N~2~-[(2R)-2-benzyl-3-(tert-butylsulfonyl)propanoyl]-N-{(1R)-1-(cyclohexylmethyl)-3,3-difluoro-2,2-dihydroxy-4-[(2-morpholin-4-ylethyl)amino]-4-oxobutyl}-3-(1H-imidazol-3-ium-4-yl)-L-alaninamide 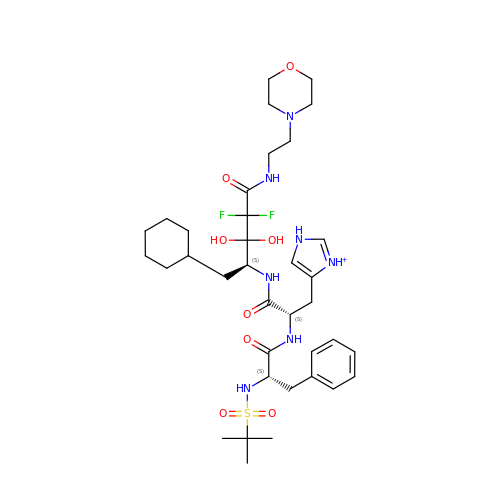| C36 H56 F2 N7 O8 S | RRJUDVVMLCYZDV-DTXPUJKBSA-O> MENGYTYEDYKNTAEWLLSHTKHRPQVAIICGSGLGGLTDKLTQAQIFDYSEIPNFPRSTVPGHAGRLVFGFLNGRACVMMQGRFHMYEGYPLWKVTFPV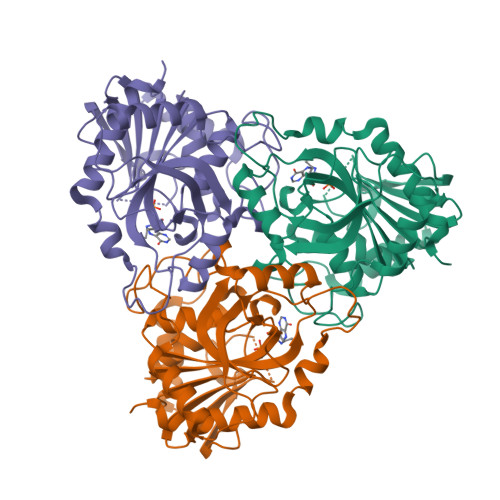RVFHLLGVDTLVVTNAAGGLNPKFEVGDIMLIRDHINLPGFSGQNPLRGPNDERFGDRFPAMSDAYDRTMRQRALSTWKQMGEQRELQEGTYVMVAGPSFETVAECRVLQKLGADAVGMSTVPEVIVARHCGLRVFGFSLITNKVIMDYESLEKANGEEVLAAGKQAAQKLEQFVSILMASIPLPDKAS> GPLGSHMSVYPKALRDEYIMSKTLGSGACGEVKLAFERKTCKKVAIKIISKRKFAIGSAREADPALNVETEIEILKKLNHPCIIKIKNFFDAEDYYIVLELMEGGELFDKVVGNKRLKEATCKLYFYQMLLAVQYLHENGIIHRDLKPENVLLSSQEEDCLIKITDFGHSKILGETSLMRTLCGTPTYLAPEVLVSVGTAGYNRAVDCWSLGVILFICLSGYPPFSEHRTQVSLKDQITSGKYNFIPEVWAEVSEKALDLVKKLLVVDPKARFTTEEALRHPWLQDEDMKRKFQDLLSEENESTALPQVLAQPSTSRKRPREGEAEGAE

Checkpoint kinase 2 (CHK2) is a serine/threonine kinase crucial in the activation of signal transduction pathways involved in the cellular response to DNA damage caused by external agents. In response to double strand DNA breaks, CHK2 is activated through initial phosphorylation on Thr68 by the DNA damage sensor ataxia-telangiectasia mutated (ATM) and subsequent trans-autophosphorylation on Thr383 and Thr387 and cis-autophosphorylation on Ser516. In its fully activated state CHK2 is known to phosphorylate a variety of substrates involved in DNA-repair, cell cycle control and apoptosis. In addition, we present the protein-ligand crystal structures of nine fragment hits, all of which bind to the hinge in the CHK2 ATP-binding site.

The binding of compound 11, which is the top-ranking hit in both the AlphaScreen™ kinase and thermal shift assays, is complicated as it can adopt different tautomers. Thus, compound 11 interacts with the hinge either through hydrogen bonds with the backbone carbonyl of Glu302 and the backbone amide of Met304, or via hydrogen bonds of both the backbone amide and carbonyl groups of Met304. Unfortunately, the structural data do not allow discrimination between these possibilities and it may even be the case that a mixture of tautomers is present in the crystal. In addition to the interactions with the hinge region, compound 11 interacts via a mediating water molecule with the side-chain hydroxyl of Thr367, located at the start of the activation loop just before the DFG motif. Furthermore, the interaction with the side chain of Thr367 observed with compounds 11 and 14 (water-mediated) and compound 12 (direct) is also found in a series of potent benzimidazole-based CHK2 inhibitors, such as 2-(4-((1-benzylpiperidin-4-yl)methoxy)phenyl)-1H-benzo[d]imidazole-5-carboxamide (5).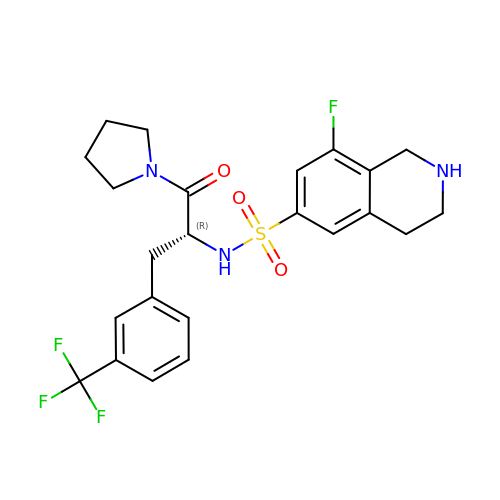8-fluoro-N-{(2R)-1-oxo-1-(pyrrolidin-1-yl)-3-[3-(trifluoromethyl)phenyl]propan-2-yl}-1,2,3,4-tetrahydroisoquinoline-6-sulfonamide | C23 H25 F4 N3 O3 S | JCKGSPAAPQRPBW-OAQYLSRUSA-N2-(1-{[2-(5-fluoro-1H-indol-4-yl)-4-(morpholin-4-yl)pyrido[3,2-d]pyrimidin-6-yl]methyl}piperidin-4-yl)propan-2-ol 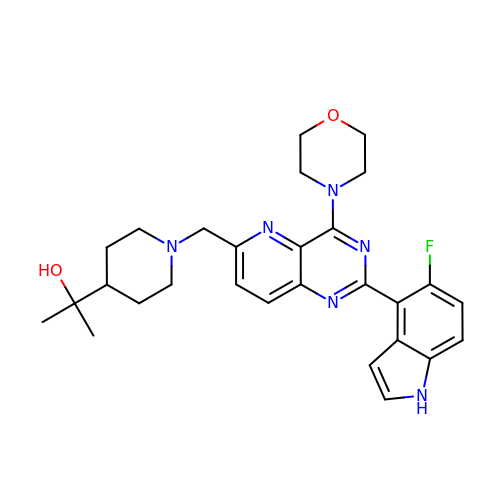| C28 H33 F N6 O2 | ONEJEIKQLAZPNN-UHFFFAOYSA-N> MELPADALPGEGAVREVLRPLLKQAAEKTAAGKIVFAEAATGTGKGRMIASLAAAAAIKGDTVVVSAPLAVTWQLVNDMKDIPEVRRVGLTLSLGRPNFISPQRTLEWAIDNERADLAAWIEGGGKPLSLRSMETSKVISHELCWLLEDALLLAEDLPADSLLLTSEDPADCPAQQLYVAMRSNYTEAGIILCSHFMLAAHTRMMQMRGLGNDEELDDEAPTGLSLPHFIDTLIVDEAHLLEQAFASVYTHTLRLRPLMRTIEGLGSRGRKPALDALKELFTQMQVASARSTNTSLNVPLSDVPELIPALKDTVKTLGALPTKGMSRDARSVIRIATRAANDALSGHSRLRIEVTPVHSYPMLLSGRSNLQRALLGLWNATGGATLVSATLFTTGDNGSLTRWKLEVPTERAAFLPPVHPAWTT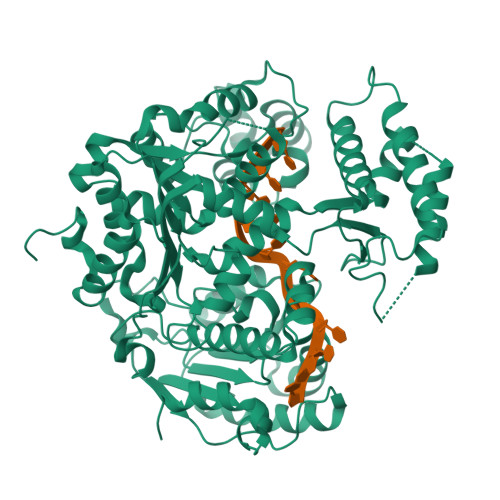APVLLHKEFCAHEPDDSPEWATECAQTIQGVASTAQGGTLVLCTSYQNTELLAGRLGAALGDRLIVQSKTSSAATCLAQFKAKHKAGIRPVWLGLGAAWTGIDLSDHSLPDNPELDRLLSDLVITRIPVGQNRSLTHERRTAIGGFRIISQEAAWHFRQGLGRLVRRPGVTHKNLWVLDARIYGGAAWVAPFRQILDRYKKA> MASRLFGVKCHNTDSEPLKNEDLLKNLLTMGVDIDMARKRQPGVFHRMITNEQDLKMFLLSKGASKEVIASIISRYPRAITRTPENLSKRWDLWRKIVTSDLEIVNILERSPESFFRSNNNLNLENNIKFLYSVGLTRKCLCRLLTNAPRTFSNSLDLNKQMVEFLQAAGLSLGHNDPADFVRKIIFKNPFILIQSTKRVKANIEFLRSTFNLNSEELLVLICGP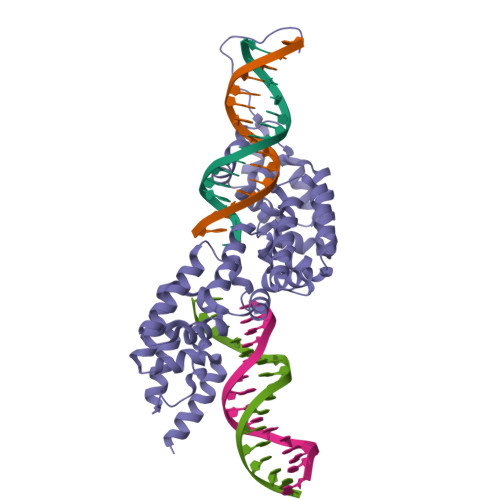GAEILDLSNDYARRSYANIKEKLFSLGCTEEEVQKFVLSYPDVIFLAEKKFNDKIDCLMEENISISQIIENPRVLDSSISTLKSRIKELVNAGCNLSTLNITLLSWSKKRYEAKLKKLSRFAHHHHHH N,N'-(6,6'-dihydroxybiphenyl-3,3'-diyl)diacetamide | C16 H16 N2 O4 | 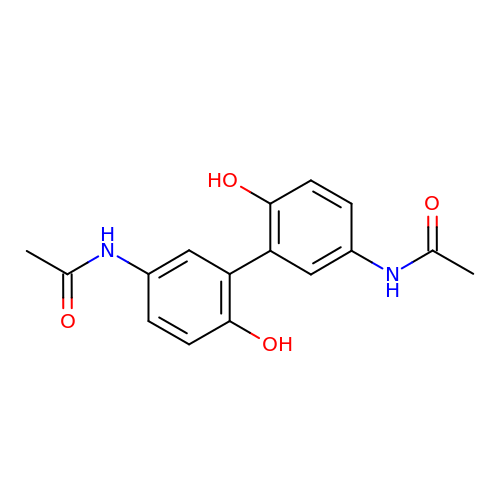PHJCCQZHFLRCAA-UHFFFAOYSA-N2,3-dihydroxanthosine | C10 H12 N4 O6 | 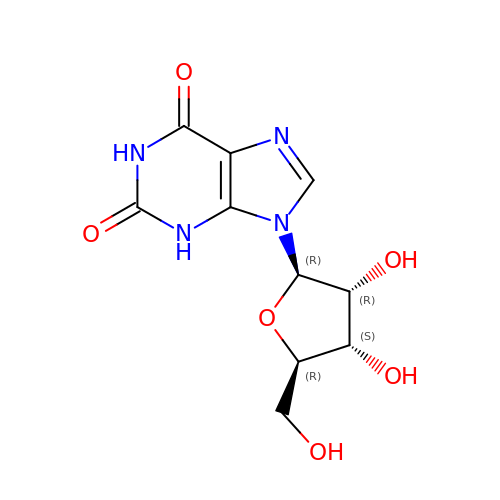UBORTCNDUKBEOP-UUOKFMHZSA-N>MTSLEIAIIVAIVLVIAIAVGWYLYTTFAAAGQQTGLTATKATIYVTKDGNVYLNVTLVPQGAAQVAISSIEVAGVSI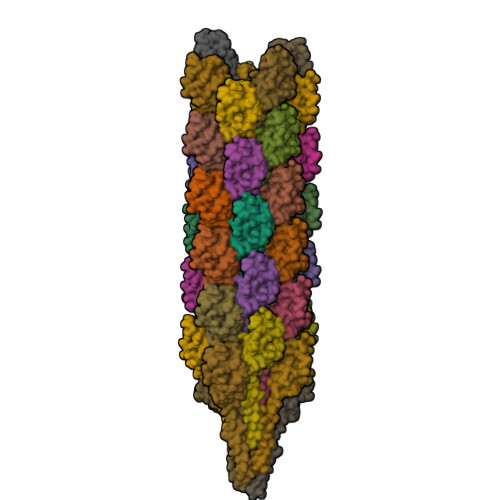PCTSSNLVKAPGEYVIELSSVSVSVGQVLTGRIVLASGAISPFTATVVAADHVPSTENKLCSSQ[41x]> GMTASTAPQTEPHKTSAPESGPVMLLVATIKGAWFLASDPARRTWELRGPVFLGHTIHHIVQDPREPERMLMAARTGHLGPTVFRSDDGGGNWTEATRPPAFNKAPEGETGRVVDHVFWLTPGHASEPGTWYAGTSPQGLFRSTDHGASWEPVAGFNDHPMRRAWTGGEQDGTPDGPKMHSILVDPRDPKHLYIGMSSGGVFESTDAGTDWKPLNRGCAANFLPDPNVEFGHDPHCVVQHPAAPDILYQQNHCGIYRMDRREGVWKRIGDAM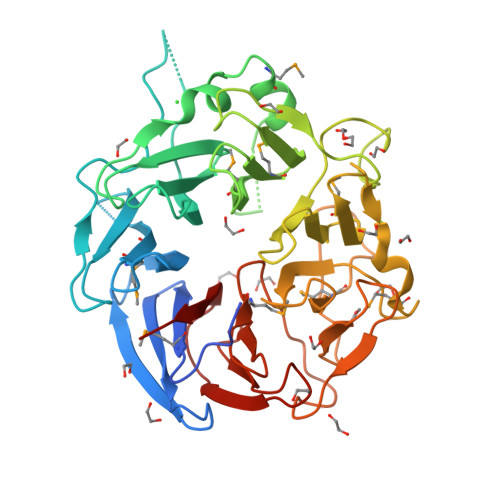PREVGDIGFPIVVHQRDPRTVWVFPMDGSDVWPRVSPGGKPAVYVTRDAGESWQRQDRGLPTDQAWLTVKRQAMTADAHAPVGVYFGTTGGEIWASADEGEHWQCIASHLPHIYAVQSARPV(2S)-2-[3-(AMINOMETHYL)PHENYL]-3-{(R)-HYDROXY[(1R)-2-METHYL-1-{[(3-PHENYLPROPYL)SULFONYL]AMINO}PROPYL]PHOSPHORYL}PROPANOIC ACID | C23 H33 N2 O6 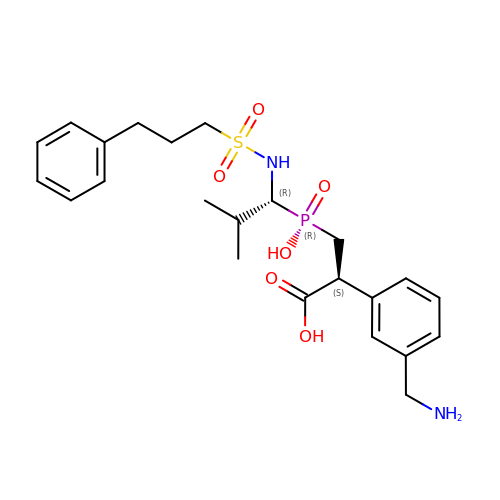P S | WFFOOKSVFDUPDH-FCHUYYIVSA-N>MALAKIVFASMTGNTEEIADIVADKLRDLGLDVDVDECTTVDASDFLEADIAIVATYTYGDGELPDEMMDFYEDLADLNLNGKIYGVVGSGDTFYDEFCKAVDDFDRVFVSTGAEKGSECVKVDLSAEEEDIERLEQFAEELAAKVGA[2x]

Flavodoxins are electron transfer proteins that participate in a variety of reactions in prokaryotes and in some unicellular algae. The identification of flavodoxin as an essential protein for S. pneumoniae infectivity and the fact that flavodoxin is not present in humans open the possibility of using it as a target for the development of novel and specific antimicrobials against S. pneumoniae. According to its gene sequence translation, it contains 147 residues and very likely belongs to the so-called short-chain flavodoxins characterized by the lack of a 20-residue loop that, in the long-chain flavodoxins, appears intercalated in the fifth β-strand. Either structure shows the archetypical α/β sandwich flavodoxin fold (5 α-helices that pack against a five-stranded β-sheet with a 21345 topology, forming an α/β/α sandwich).

To understand the molecular basis of the interaction of the FMN cofactor with the protein moiety and to provide a structural frame for the identification and characterization of SpFld inhibitors, we have solved the crystal structures of the SpFld in the apo form and in complex with FMN, at 2.18 and 1.69 Å, respectively. Overall, the holo (note that the holo form contains selenomethionine (SeMet) residues) and apo SpFld structures are similar with an r.m.s.d of 0.8 Å. The main differences between the two structures are traced to two of the three FMN binding loops encompassing residues 10–14 (phosphate loop), 57–66 (50’ loop) and 92–100 (90’ loop), the latter two sandwiching the isoalloxazine moiety. A further noticeable difference is the presence of a small 310 helix stretch at residues 38–40 in the holoprotein that is absent in the apo form. In its bound conformation, the FMN phosphate group forms hydrogen bonds with S10 (sc), M11 (N), T12 (sc and N), N14 (N) and T15 (sc and N). As previously reported for the apo/holo flavodoxin pairs in Anabaena PCC7119 and H. pylori, the entrance of the FMN cofactor makes the two isoalloxazine binding loops to move apart. In this reorganization, existing interactions between the two loops in the apoform (Y95/G60 and E97/G62) are broken and the protein expands: the holoprotein surface area is 7745 Å compared to 7135 Å for the apoprotein. In the holoprotein, FMN is embedded by Y59, D92, E97, Y95, C99 and G60. The isoalloxazine ring of FMN establishes π-π interactions with Y59 and Y95. The dissociation constant at 25°C is 83 nM, not far from that of Helicobacter pylori flavodoxin (27 nM), but two orders of magnitude higher than that of Anabaena flavodoxin (0.26 nM).> MVATTSSGGSSVGWPSRLSGVRLHLVTGKGGTGKSTIAAALALTLAAGGRKVLLVEVEGRQGIAQLFDVPPLPYQELKIATAERGGQVNALAIDIEAAFLEYLDMFYNLGIAGRAMRRIGAVEFATTIAPGLRDVLLTGKIKETVVRLDKNKLPVYDAIVVDAPPTGRIARFLDVTKAVSDLAKGGPVHAQSEGVVKLLHSNQTAIHLVTLLEALPVQETLEAIEELAQMELPIGSVIVNRNIPAHLEPQDLAKAAEGEVDADSVRAGLLTAGVKLPDADFAGLLTETIQHATRITARAEIAQQLDALQVPRLELPTVSDGVDLGSLYELSESLAQQGV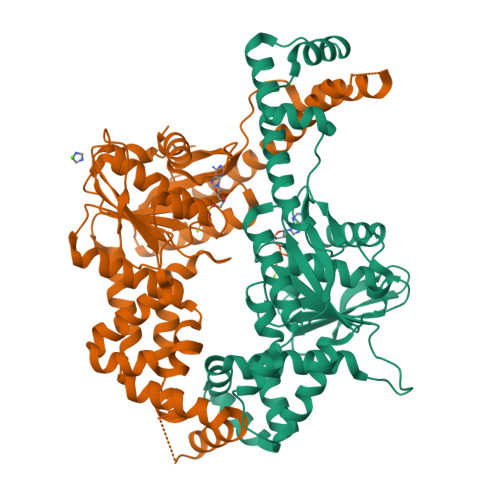R;> MSVTPKTLDMGAILADTSNRVVVCCGAGGVGKTTTAAALALRAAEYGRTVVVLTIDPAKRLAQALGINDLGNTPQRVPLAPEVPGELHAMMLDMRRTFDEMVMQYSGPERAQSILDNQFYQTVATSLAGTQEYMAMEKLGQLLSQDRWDLIVVDTPPSRNALDFLDAPKRLGSFMDSRLWRLLLAPGRGIGRLITGVMGLAMKALSTVLGSQMLADAAAFVQSLDATFGGFREKADRTYALLKRRGTQFVVVSAAEPDALREASFFVDRLSQESMPLAGLVFNRTHPMLCALPIERAIDAAETLDAETTDSDATSLAAAVLRIHAERGQTAKREIRLLSRFTGANPTVPVVGVPSLPFDVSDLEALRALADQLTTVGNDAGRAAGRLEHHHHHH> MSQAALNTRNSEEEVSSRRNNGTRLAGILFLLTVLTTVLVSGWVVLGWMEDAQRLPLSKLVLTGERHYTRNDDIRQ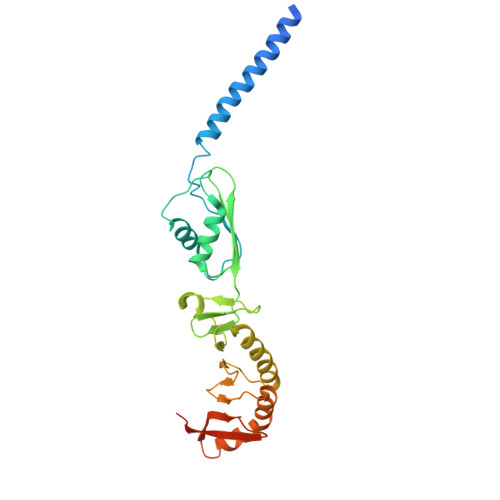SILALGEPGTFMTQDVNIIQTQIEQRLPWIKQVSVRKQWPDELKIHLVEYVPIARWNDQHMVDAEGNTFSVPPERTSKQVLPMLYGPEGSANEVLQGYREMGQMLAKDRFTLKEAAMTARRSWQLTLNNDIKLNLGRGDTMKRLARFVELYPVLQQQAQTDGKRISYVDLRYDSGAAVGWAPLPPEESTQQQNQAQAEQQ> MLFPDDYTKTPYIPVYASLPMGIINSHCQLVDPESVRAELRQLKSLNVDGVVVDCWWGIVEAWTPRKYEWSGYRDLFGIIKEFKLKVQVVLSFHGSGETGSGDVLISLPKWIMEIAKENQDIFFTDREGRRNTECLSWGIDKERVLRGRTGIEVCFDFMRSFHMEFRNLSEEGLVSSIEIGLGASGELRYPSCPETMGWKYPGIGEFQCYDRYMQKNLRQSALSRGHLFWARGPDNAGYYNSRPHETGFFCDGGDYDSYYGRFFLN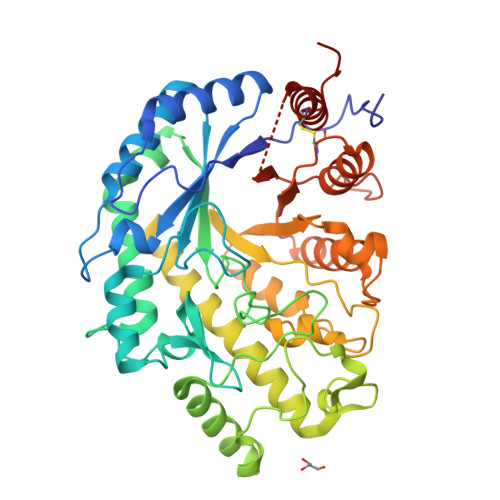WYSGVLMDHVDQVLSLATLAFDGAEIVVKVPSIYWWYRTASHAAELTAGFYNTTNRDGYSPVFRMLKKHSVILKLVCYGPEYTVHEKDDDEAFADPEGLTWQVINAAWDQGLPLCIESALPCRNGEAYSRILDTAKPRDDPDRHHAASFAYRQQQQPPLREACLSELCTFVKCMHGEAPQNGEG(2S)-1-[[(1R,5S)-3-azabicyclo[3.1.0]hexan-3-yl]carbonyl]-N-(2-cyclopropylethyl)-2-methyl-4-oxidanylidene-3,5-dihydro-2H-1,5-benzodiazepine-7-carboxamide 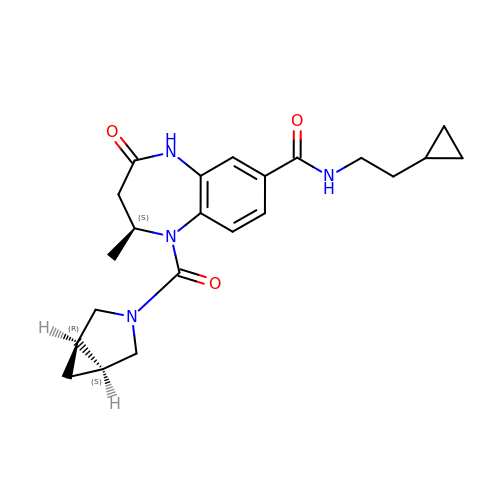| C22 H28 N4 O3 | CKFRXCBNKKOFGO-RRQGHBQHSA-N> MHHHHHHLVPRGSNRDILRTLSLKGDHNIRVAILDGPVDIAHPCFQGADLTVLPTLAPTAARSDGFMSAHGTHVASIIFGQPETSVPGIAPQCRGLIV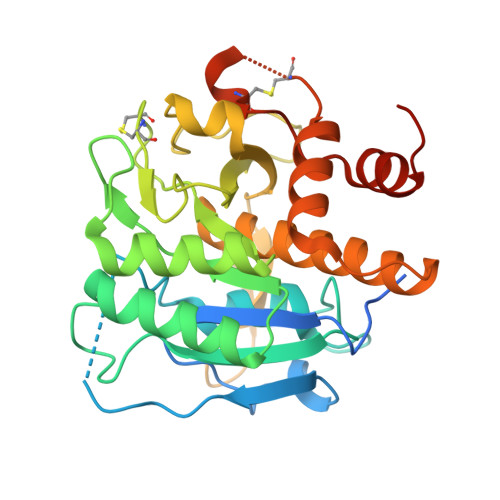PIFSDDRRRITQLDLARGIERAVNAGAHIINISGGELTDFGEADGWLENAVSLCRQNNVLLVAAAGNNGCDCLHVPAALPAVLAVGAMDDHGHPLDFSNWGSTYEQQGILAPGEDILGAKPGGGTERLSGTSFATPIVSGVAALLLSEQVRRGETPDPQKVRQLLLQSALPCDDDAPEQARRCLAGRLNVSGAFTLLKGGNMSEELATA>[4x]MNVSAESGAPRRAGQRHEVGLAQLPPAPPTTVAVIEGLATGTPRRVVNQSDAADRVAELFLDPGQRERIPRVYQKSRITTRRMAVDPLDAKFDVFRREPATIRDRMHLFYEHAVPLAVDVSKRALAGLPYRAAEIGLLVLATSTGFIAPGVDVAIVKELGLSPSISRVVVNFMGCAAAM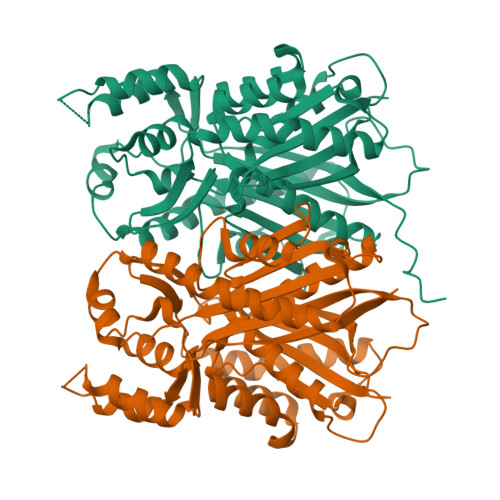NALGTATNYVRAHPAMKALVVCIELFSVNAVFADDINDVVIHSLFGDGCAALVIGASQVQEKLEPGKVVVRSSFSQLLDNTEDGIVLGVNHNGITCELSENLPGYIFSGVAPVVTEMLWDNGLQISDIDLWAIHPGGPKIIEQSVRSLGISAELAAQSWDVLARFGNMLSVSLIFVLETMVQQAESAKAISTGVAFAFGPGVTVEGMLFDIIRR>[2x]ANSGEAPKNFGLDVKITGESENDRDLGTAPGGTLNDIGIDLRPWAFGQWGDWSAYFMGQAVAATDTIETDTLQSDTDDGNNSRNDGREPDKSYLAAREFWVDYAGLTAYPGEHLRFGRQRLREDSGQWQDTNIEALNWSFETTLLNAHAGVAQRFSEYRTDLDELAPEDK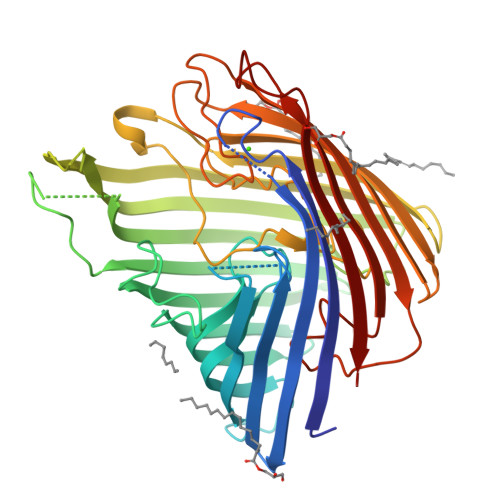DRTHVFGDISTQWAPHHRIGVRIHHADDSGHLRRPGEEVDNLDKTYTGQLTWLGIEATGDAYNYRSSMPLNYWASATWLTGDRDNLTTTTVDDRRIATGKQSGDVNAFGVDLGLRWNIDEQWKAGVGYARGSGGGKDGEEQFQQTGLESNRSNFTGTRSRVHRFGEAFRGELSNLQAATLFGSWQLREDYDASLVYHKFWRVDDDSDIGTSGINAALQPGEKDIGQELDLVVTKYFKQGLLPASMSQYVDEPSALIRFRGGLFKPGDAYGPGTDSTMHRAFVDFIWRF> ESEKQQWFCNSSDAIISYSYCDHLK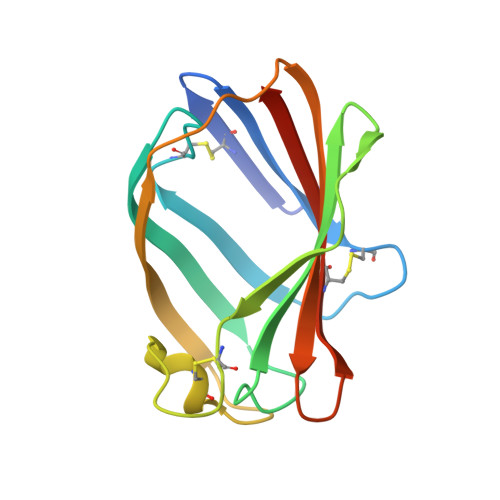FPISISSEPCIRLRGTNGFVHVEFIPRGNLKYLYFNLFISVNSIELPKRKEVLCHGHDDDYSFCRALKGETVNTSIPFSFEGILFPKGHYRCVAEAIAGDTEEKLFCLNFTIIHRRDVN>GS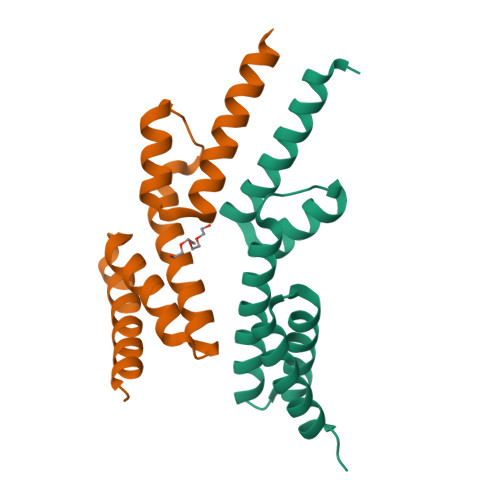HMNLAVKLTRMEKTLKAYELYIFSDYENFENYVKKEGLKIEGMELLKEKKARSLIAEGKDLFETANYGEALVFFEKALNLSDNEEIKKIASFYLEECRKKLAGD[4x]> MASHKLLVTPPKALLKPLSIPNQLLLGPGPSNLPPRIMAAGGLQMIGHMSKEMYQIMDEIKEGIQYVFQTRNPLTLVISGSGHCALEAALVNVLEPGDSFLVGANGIWGQRAVDIGERIGARVHPMTKDPGGHYTLQEVEEGLAQHKPVLLFLTHGESSTGVLQPLDGFGELCHRYKCLLLVDSVASLGGTPLYMDRQGIDILYSGSQKALNAPPGTSLISFSDKAKKKMYSRKTKPFSFYLDIKWLANFWGCDDQPRMYHHTIPVISLYSLRESLALIAEQGLENSWRQHREAAAYLHGRLQALGLQLFVKDP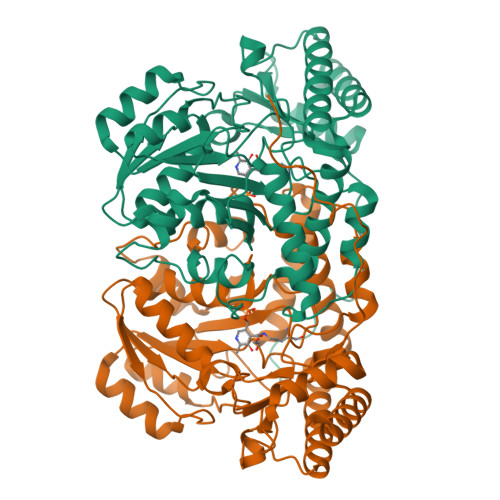ALRLPTVTTVAVPAGYDWRDIVSYVMDHFDIEIMGGLGPSTGKVLRIGLLGCNATRENVDRVTEALRAALQHCPKKKL Tom1p is a large, 374 kDa member of a broadly conserved family of HUWE1 factors (also called Mule, Lasu, Ureb1, Arf-BP1, HectH9/E3^Histone^, Ptr1, Upl1, or Eel-1;). This family is characterized by a large N-terminal domain attached to a smaller C-terminal HECT domain (Homologous to E6-AP Carboxyl Terminus) that provides ubiquitin ligase activity ([Fig fig1]). Tom1p has been implicated in the turnover of excess levels of small, basic proteins including ribosomal components and histones. We determined cryo-EM structures of Tom1p to reveal a helical repeat solenoid architecture for the 2,888 residues preceding the C-terminal HECT domain and an overall architecture that resembles the published structures of HUWE1 but with a larger fraction of ordered residues.

HECT domains comprise two lobes, an N-terminal lobe and a smaller C-terminal lobe that houses the catalytic cysteine residue (C3235 in Tom1p). Multiple HECT domain crystal structures have indicated that the two lobes rotate with respect to each other through the catalytic cycle of binding E2, transthiolation of ubiquitin from E2 to the HECT domain cysteine, and subsequent ubiquitylation of substrate. The 379-residue HECT domain adopts similar structures and maintains the same intramolecular contacts in the open and closed solenoid structures of Tom1p and in the published structures of human and *Nematocida* HUWE1. Overlap of the Tom1p and human HUWE1 HECT domains shows a 1.1 Å RMSD over 256 pairs of Cα atoms. The HECT domains of Tom1p/HUWE1 family members are thought to ubquitylate substrates, likely for subsequent degradation by the proteasome, while more N-terminal sequences presumably function in substrate recognition.

> NLFFPFTDAHKKLLNQMIRSNPKLMSGPFALLVKNQKVLDFDNKRYFFNAKLKSDNQERPKLPITVRREQVFLDSYRALFFKTNDEIKNSKLEITFKGESGVDAGGVTREWYQVLSRQMFNPDYALFLPVPSDKTTFHPNRTSALNPEHLSFFKFIGMIIGKAIRDQCFLDCHFSREVYKNILGRPVSLKDMESLDPDYYKSLVWILENDITDIIEETFSVETDDYGEHKVINLIEGGKDIIVTEANKQDYVKKVVEYKLQTSVKEQMDNFLVGFYALISKDLITIFDEQELELLISGLPDIDVDDWKNNTTYVNYTATCKEVSYFWRAVRSFDAEERAKLLQFVTGTSKVPLNGFKELSGVNGVCKFSIHRDFGSSERLPSSHTCFNQLNLPPYESYETLRGSLLLAINEG>MTDEKKVPSKPARPARKPRADKPADAKPAAVPKVAAPAVVEGSSTNAAAVKKSLRDGGMTALPSEILFAVGSIPLVVDKDALSTLAAALVASDDPSTWFVANRELIRAVVFVPQQNNVLRATPLLSVRPVASLSSVHNWQVRNHLSGLHVVVGGTGAGKSKWLNAQTPDVTIRWGEPGETFDMEESSIAVADLTEMLAVALLLATADYRVVIDSFRNLVFGITGAAGPGGVSVALYAALTSLNNICAELGVLLVAAINPMSSDDKVSLVYNNIAASVAGMTVVNNAAVVSQTIRSGTGRIFSGEPAPRNDSPVEYHEPRHTQLDEPSGPSARIRLESNNIDPDDENDNRPRRGARIS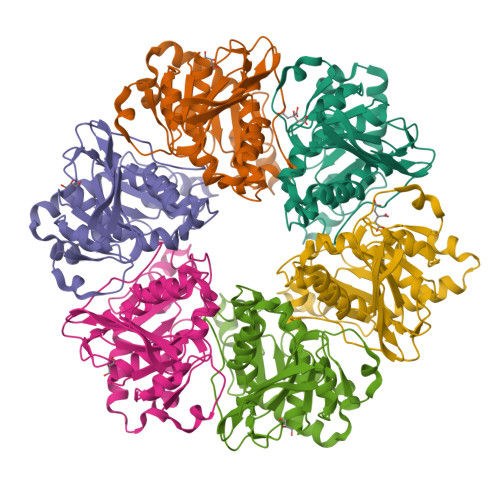L[6x]trihydroxy(octyl)borate(1-) 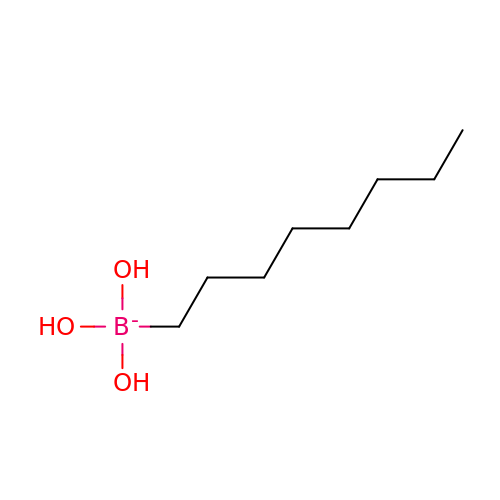| C8 H20 B O3 | UFILDBLRNSLDDP-UHFFFAOYSA-N> TLESVKDECQPGVDFPHNPLATCHTYVIKRVCGRGPSRPMLVKERCCRELAAVPDHCRCEALRILMDG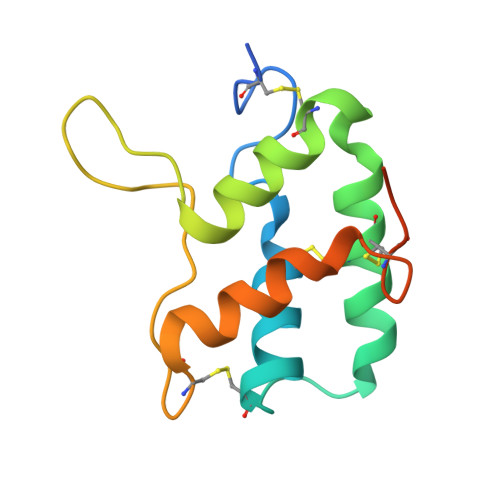VRTPEGRVVEGRLGDRRDCPREEQRAFAATLVTAAECNLSSVQEPGHHHHHH> GSAMGMSNTQAERSIIGMIDMFHKYTRRDGKIDKPSLLTMMKENFPNFLSACDKKGTNYLADVFEKKD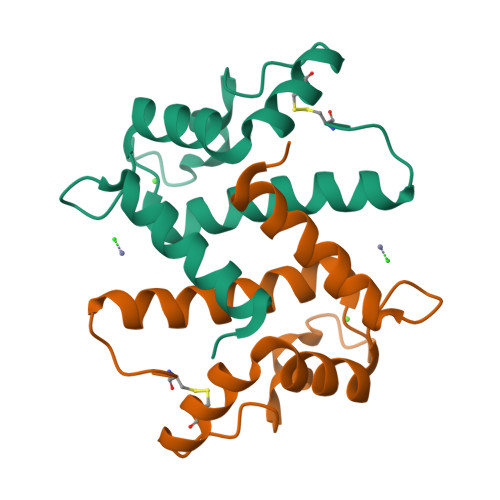KNEDKKIDFSEFLSLLGDIATDYHKQSHGAAPCSGGSQAAA5-N-acetyl-4-amino-6-diethyl carboxamide-4,5-dihydro-2H-pyran-2-carboxylic acid | C13 H21 N3 O5 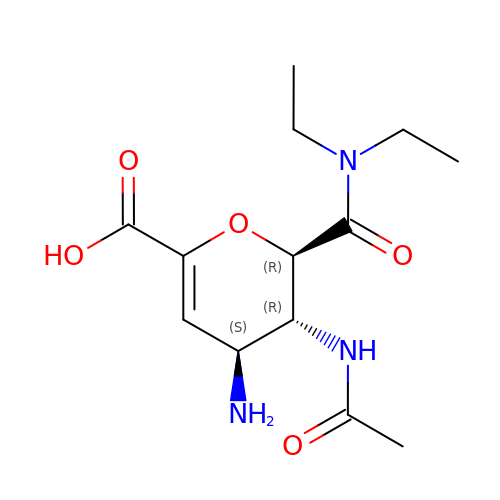| YQUCNOUQEZHVSC-JMJZKYOTSA-N>[2x]AVTGPPPPLSHCGRAAPCEPLRYNVCLGSVLPYGATSTLLAGDSDSQEEAHGKLVLWSGLRNAPRCWAVIQPLLCAVYMPKCENDRVELPSRTLCQATRGPCAIVERERGWPDFLRCTPDRFPEGCTNEVQNIKFNSSGQCMVPLVRTDNPKSWYEDVEGCGIQCQNPLFTEAEHQDMHSYIAAFGAVTGLCTLFTLATFVADWRNSNRYPAVILFYVNACFFVGSIGWLAQFMDGARREIVCRADGTMRLGEPTSNETLSCVIIFVIVYYALMAGVVWFVVLTYAWHTSFKALGTTYQPLSGKTSYFHLLTWSLPFVLTVAILAVAQVDGDSVSGICFVGYKNYRYRAGFVLAPIGLVLIVGGYFLIRGVMTLFSIKSNHAKALIVYGSTTGNTEYTAETIARELADAGYEVDSRDAASVEAGGLFEGFDLVLLGCSTWGDDSIELQDDFIPLFDSLEETGAQGRKVACFGCGDSSWEYFCGAVDAIEEKLKNLGAEIVQDGLRIDGDPRAARDDIVGWAHDVRGAIKINETMLRLGIFGFLAFGFVLITFSCHFYDFFNQAEWERSFRDYVLCQANVTIGLPTKQPIPDCEIKNRPSLLVEKINLFAMFGTGIAMSTWVWTKATLLIWRRTWCRLTGQSDDHHHHHHHHHH

The smoothened receptor (SMO), a Class Frizzled seven-transmembrane helices (7TM) G protein-coupled receptor (GPCR), is a key component in this signalling pathway. The activity of SMO is suppressed by the PTCH receptor, a 12TM protein. This suppression is disabled when Hh binds to PTCH, leading to phosphorylation of SMO's cytoplasmic region5, which induces the translocation of GLI transcription factors into the nucleus to activate target genes. Here, we present the crystal structure of the multi-domain human SMO in complex with a specially designed TMD ligand, shedding light on interactions between the CRD and TMD.

To facilitate crystallization, human SMO was engineered by fusion of a Flavodoxin (FLA)16 protein between helices V and VI, replacing part of intracellular loop 3 (ICL3) between P434 and S443. The N terminus 1–52 and C terminus 559–787 were truncated and a single-mutation E194M was made in the hinge domain (HD), which slightly increased the protein yield without affecting its stability compared to the construct without this mutation. The resulting SMO–FLA construct was co-expressed with vismodegib, and then purified and crystallized in complex with TC114 using the lipidic cubic phase method. We determined the structure using room temperature data collected at an X-ray free-electron laser (XFEL) source at 2.9 Å resolution. Since the room temperature XFEL crystal structure potentially represents a closer-to-native receptor conformation and at a slightly higher resolution than the synchrotron structure obtained at cryo-cooled conditions, we describe the XFEL SMO structure below, unless noted otherwise. Analysis of our multi-domain SMO structures indicated that the nitro group introduced in the TC114 ligand does interact strongly with K395 in SMO as designed, and enhance the π–π stacking between the benzoyl group and F484 on helix VI. The CRD is positioned straight up on top of the TMD and is supported by extracellular loop 3 (ECL3) on one side and by a linker loop (residues 181–190) on the other. Furthermore, on the extracellular side of the structure, helix VI is extended beyond the membrane surface by four α-helical turns, and the top part of helix VI is tilted at a non-proline kink towards the CRD, protruding into its hydrophobic groove and bridging a key connection between the CRD and TMD. In the vismodegib-bound structure, the glycan partially occupies the cholesterol binding site precluding cholesterol or oxysterol binding to the vismodegib-bound structure, whereas in our XFEL structure the side chain of I496 from ECL3 extends into the cholesterol binding site, also precluding cholesterol or oxysterol binding to the CRD. In fact, our structure demonstrates that in the absence of sterol binding, ECL3 interacts with the CRD hydrophobic groove to stabilize the CRD in a ‘closed' conformation.>[2x]SGGKLTAVDPETNMNVSEIISYWGFPSEEYLVETEDGYILCLNRIPHGRKQHSDKGPKPVVFLQHGLLADSSNWVTNLAQSSLGFILADA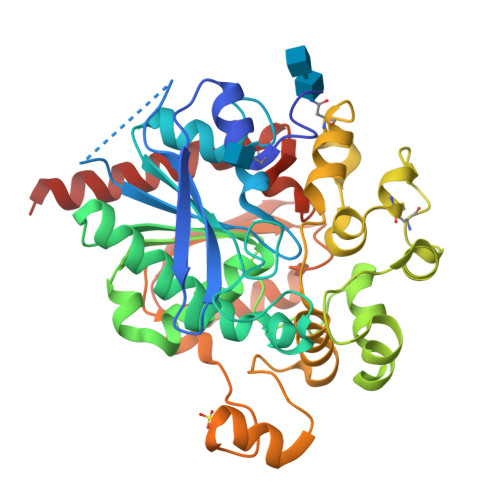GFDVWMGNSRGNTWSRKHKTLSVSQDEFWAFSYDEMAKYDLPASINFILNKTGQEQVYYVGHSQGTTIGFIAFSQIPELAKRIKMFFALGPVASVAFCTSPMAKLGRLPDHLIKDLFGDKEFLPQSAFLKWLGTHVCTHVILKELCGNLCFLLCGFNERNLNMSRVDVYTTHSPAGTSVQNMLHWSQAVKFQKFQAFDWGSSAKNYFHYQQSYPPTYNVKDMLVPTAVWSGGHDWLADVYDVNILLTQITNLVFHESIPEWEHLDFIWGLDAPWRLYNKIINLMRKYQASENNL> HMMENINIVIKDVGYFQDKPQFLNSKSVR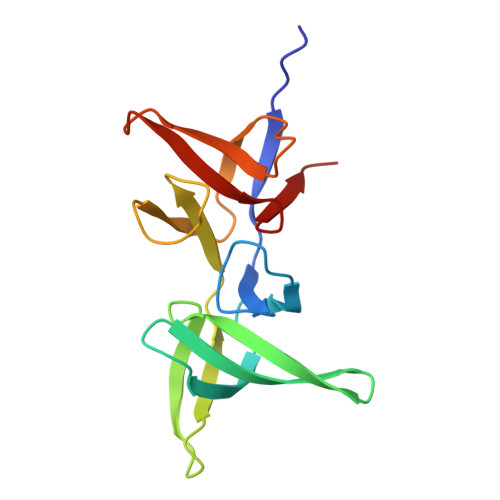QWKHGTKVKLTKHNSHWYTGVVKDGNKSVRGYIYHSMAKVTSKNSDGSVNATINAHAFCWDNKKLNGGDFINLKRGFKGITHPASDGFYPLYFASRKKTFYIPRYMFDIKG>FSEECMHGSGENYDGKISKTMSGLECQAWDSQSPHAHGYIPSKFPNKNLKKNYCRNPDRDLRPWCFTTDPNKRWEYCDIPRCAA[2x];>[2x]VEKLTADAELQRLKNERHEEAELER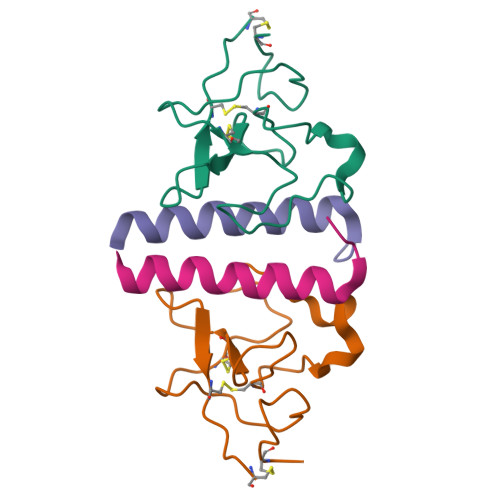LKSEY>[2x]SNAEAKSIEDTNMASCITNKKFVQLEKKFDARLGVYAIDIGSNKTIAYRPNERFAYASTYKVLAAAAVLKKNSIEKLNEVIHYSKDDLVTYSPITEKHLDTGMSLKEISEAAIRYSDNTAG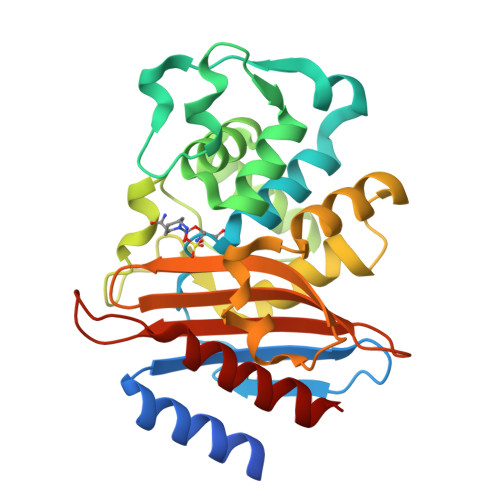NILLQQLGGPKGFEKSLKQIGDHVTKAKRFETDLNSAIPGDIRDTSTAKALATDLKAFTLDNTLTTDKRMILTDWMRGNATGDELIRAGAPIGWEVGDKSGAGSYGTRNDIAIVWPPNRAPIVVAILSNRFTKDANYDNALIAEAAKVVLNDLK> GIEETIDTVITNALQLSQPKPQKQPTAQSTPLTSGVNSQEVPALTAVETGASGQAVPSDVIETRHVVNYKTRSESTLESFFGRSACVTILEVENFNATTDADRKKQFTTWAITYTDTVQLRRKLEFFTYSRFDLEMTFVITERYYASNTGHARNQVYQLMYIPPGAPRPTAWDDYTWQSSSNPSVFYTYGSAPPRMSIPYVGIANAYSHFYDGFARVPLKDETVDSGDTYYGLVTINDFGTLAVRVVNEYNPARITSKIRVYMKPKHVRCWCPRPPRAVPYRGEGVDFKQDSITPLTAVENINTF;> SPNVEACGYSDRVRQITLGNSTITTQEAANAVVAYGEWPSYLDDKEANPIDAPTEPDVSSNRFYTLDSVQWKSTSRGWWWKLPDALKDMGMFGQNMYYHYLGRSGYTVHVQCNASKFHQGALGVFAIPEYVMACNTEAKTSYVSYVNANPGEKGGVFDNAYNPSAEASEGRKFAALDYLLGCGVLAGNAFVYPHQIINLRTNNSATLVLPYVNSLAIDCMAKHNNWGLVILPLCKLDYAPNSSTEIPITVTIAPMFTEFNGLRNITVPATQ;> GLPTMLTPGSSQFLTSDDFQSPCALPNFDVTPPIHIPGEVFNMMELAEIDSMIPMNSVTGKANTMEMYPIPLDDKGSATPIFSISLSPASDKRLQYTMLGEILNYYTHWTGSLRFTFLFCGSMMATGKILLSYSPPGAKPPTTRKDAMLGTHIIWDLGLQSSCTMLAPWISNTVYRRCIKDDFTEGGYITCFYQTRIVVPSGTPTSMFMLAFVSACPDFSVRLLRDTNHISQRTLFARAQ;> MGAQVSSQKVGAHENTNVATGGSTVNYTTINYYKDSASNAASKLDFSQDPSKFTEPVKDIMIKTAPALN

CVA24v attaches to cells by binding Neu5Ac-containing glycans on the surface of cells which facilitates entry. CVA24v is reported to engage receptors with terminal α2,3- and α2,6-linked Neu5Ac, with some preference for the α2,6-linkage. CVA24v attaches to cells via shallow, surface exposed, Neu5Ac pockets. The CVA24v capsid is decorated by a total of sixty individual Neu5Ac binding sites which are further arranged into twelve local five-fold symmetries (i.e. twelve regular pentagons).

As a starting point to probe this strategy, divalent Neu5Ac compounds posed as attractive tools as they have potential to bind to the virion by simultaneously occupying two Neu5Ac binding sites. The hydroxyls attached to C2 and C9 serve as promising connection points as they are pointing towards the solvent, thereby minimizing possible steric clashes with the virion, and are not key contributors to Neu5Ac binding. Compounds with a C2–C9 linkage between the two Neu5Ac entities proved more efficacious blocking CVA24v transduction than C4–C9 and C2–C2 linked compounds. To investigate the binding of compounds 16–21, we derivatized CVA24v by soaking CVA24v crystals in crystallization solution containing the corresponding compound (16 mM). The following structure determination resulted in data sets with resolutions below or around 2 Å and showed that all compounds, beside 17, bind by their Neu5Ac entity to the characterized binding site. The linker regions of all compounds seem not to interact with the capsid protein and are therefore not visible in the resolved X-ray crystal structures. A plausible reason is the C2–C9 linkage of these dimeric compounds. The C2 and C9 hydroxyls of the parent Neu5Ac molecule are pointing towards the solvent. Thus, we find it likely that the spacer unit that links the C2 position of one Neu5Ac entity to the C9 position of a second Neu5Ac entity is floating in the solvent in a non-ordered fashion rather than folding back towards the viral surface to interact with the canyon on top of the VP1 capsid protein. Thus, the divalent Neu5Ac compounds does not seem to affect the thermal stability of the CVA24v particle indicating the mechanism of inhibition is not related to CVA24v uncoating.> MWLTKLVLNPASRAARRDLANPYEMHRTLSKAVSRALEEGRERLLWRLEPARGLEPPVVLVQTLTEPDWSVLDEGYAQVFPPKPFH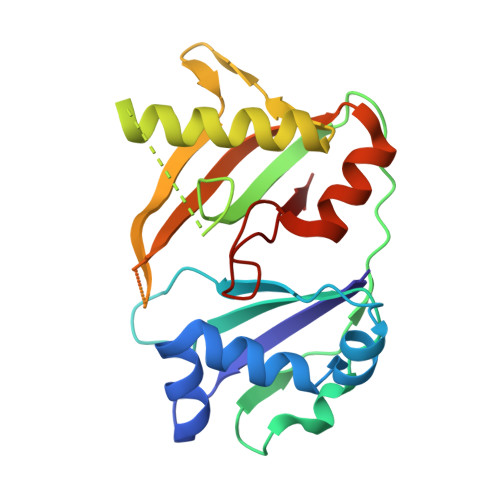PALKPGQRLRFRLRANPAKRLAATGKRVALKTPAEKVAWLERRLEEGGFRLLEGERGPWVQILQDTFLEVRRKKDGEEAGKLLQVQAVLFEGRLEVVDPERALATLRRGVGPGKALGLGLLSVAP> SGNKICQFKLVLLGESAVGKSSLVLRFVKGQFHEFQESTIGAAFLTQTVCLDDTTVKFEIWDTAGQERYHSLAPMYYRGAQAAIVVYDITNEESFARAKNWVKELQRQASPNIVIALSGNKADLANKRAVDFQEAQSYADDNSLLFMETSAKTS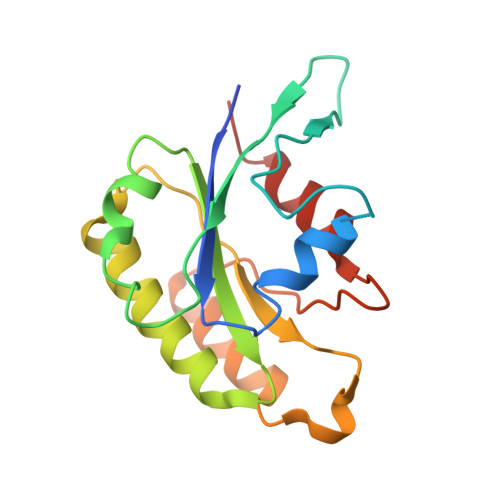MNVNEIFMAIAKKLPKN>[4x]MTELKLIHIFTDGSCLGNPGP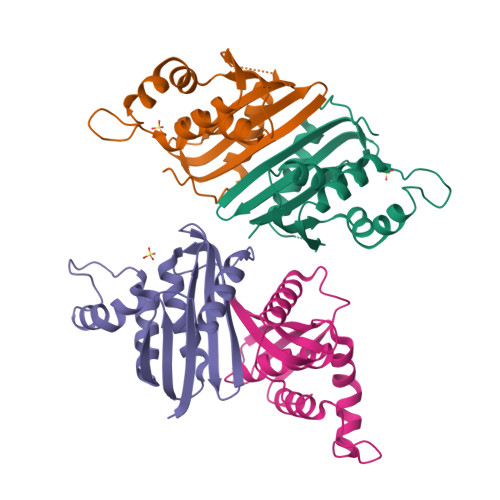GGYGIVMKYKGHTKEMSGGFSLTTNNRMELLAPIVALEALKEPCKIILTSDSQYVRQGIMTWIHGWKKNGWMTSNGTPVKNVDLWKRLDKAAQLHQIDWRWVKGHAGHAENERCHQLARAAAEANPTQIDTGYQAES>[2x]GIDPFTTRPSSDLTAFREHFAKAKHIAIITGAGVSAESGVPTFRGPGGFWRKWQAQDLATPEAFSRDPSLVWEFYHYRREVMRSKMPNPAHLAIAECEARLGQQGRSVVIITQNIDELHHRAGSKHV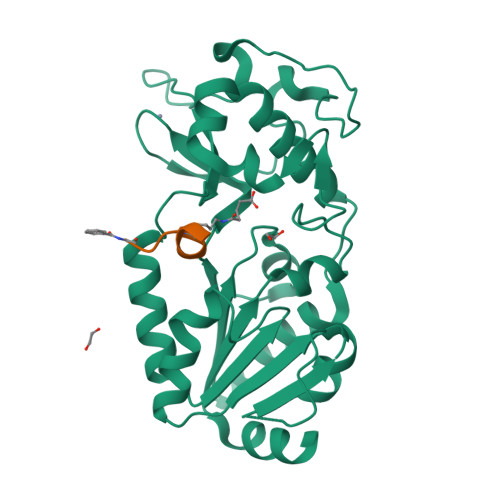YEIHGSLFKTRCMSCGEVKANHKSPICPALDGKGAPDPNTKEARIPVELLPRCERKSCNGLLRPHVVWFGETLDSDILTAVERELEKCDLCLVVGTSSIVYPAAMFAPQVASRGVPVAEFNMECTPATQRFKYHFEGPCGSTLPPALE;> XGVLKEYGV The infection cycle consists of the following steps: first, the ssRNA phage adsorbs to the side of a retractile pilus via its maturation protein (Mat), presented as a single copy in the virion shell. The capsid of MS2 is composed of a single copy of Mat and 178 coat proteins (89 coat protein dimers) with a T = 3 quasi-icosahedral symmetry. The F-pilus, the receptor for MS2, is a dynamic filament assembled by the F plasmid-encoded type IV secretion system (T4SS), which directs the conjugative transfer of F plasmids. A recent high-resolution cryo-EM structure revealed that the conjugative F-pilus is an assembly of a stoichiometric pilin-phospholipid complex forming a five-start helical filament.

To improve the resolution of the F-pilus, we created a loose mask around the F-pilus and the Mat to locally align the density within this mask. This allowed us to achieve a more uniformly resolved density of the F-pilus/Mat complex at an overall resolution of 6.2 Å. The ɑ-helices in each pilin monomer are clearly resolved, as is the internally buried phospholipid, which interacts with the ɑ2–ɑ3 loop of each F-pilin. We observe that the exposed surface of the β-sheet-rich region (or β-region) in the Mat lies parallel to the axis of the F-pilus and directly interacts with the N- and C-termini of the pilin subunits within the F-pilus in a defined manner, in which the tip of the β-region leans opposite to the N- and C-termini of the F-pilins. The area of the interface between the β-region of the Mat and the pilus is ~1062.89 Å2. At the pilus–Mat interface, residues of opposite charges have electrostatic interactions. The positively charged His357 from the Mat interacts with the Asp7 from one pilin. Two arginine residues, Arg36 and Arg99 from the Mat interact with two aspartic acids, Asp7 and Asp23, from the pilins, respectively. In contrast, in the phage-bound structure, we see extra cryo-EM density extending from the N terminus of one pilin subunit into a hydrophobic pocket (consisting of Val15, Phe31, Leu33, Phe92, and Phe94) on the exposed surface of the Mat. This electron density may correspond to the five N-terminal amino acids of a pilin subunit, which were previously missing due to their flexibility but are now stabilized by the Mat.

>QDLMASGNTTVKATFGKDSSVVKWVVLAEVLVGAVMYMMTKNVKFLAGFAIISVFIAVGMAVVGL[75x];> MRAFSTLDRENETFVPSVRVYADGETEDNSFSLKYRSNWTPGRFNSTGAKTKQWHYPSPYSRGALSVTSIDQGAYKRSGSSWGRPYEEKAGFGFSLDARSCYSLFPVSQNLTYIEVPQNVANRASTEVLQKVTQGNFNLGVALAEARSTASQLATQTIALVKAYTAARRGNWRQALRYLALNEDRKFRSKHVAGRWLELQFGWLPLMSDIQGAYEMLTKVHLQEFLPMRAVRQVGTNIKLDGRLSYPAANFQTTCNISRRIVIWFYINDARLAWLSSLGILNPLGIVWEKVPFSFVVDWLLPVGNMLEGLTAPVGCSYMSGTVTDVITGESIISVDAPYGWTVERQGTAKAQISAMHRGVQSVWPTTGAYVKSPFSMVHTLDALALIRQRLSR> GHMG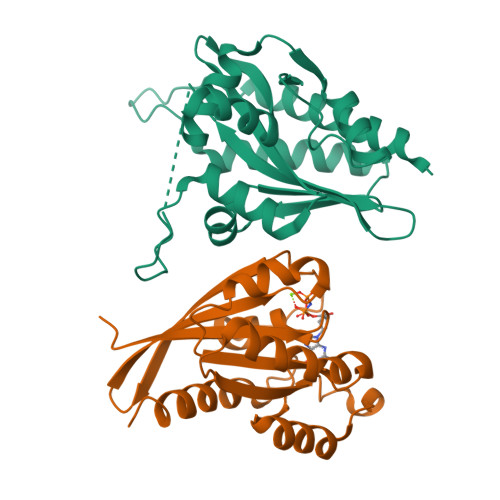QKASQQLALKDSKEVPVVCEVVSEAIVHAAQKLKEYLGFEYPPSKLCPAANTLNEIFLIHFITFCQEKGVDEWLTTTKMTKHQAFLFGADWIWTFWGSDKQIKLQLAVQTLQMSSPPPVESKPCDLSNPESRVEESSWKKSRFDKLEEFCNLIGEDCLGLFIIFGMPGKPKDIRGVVLDSVKSQMVRSHLPGGKAVAQFVLETEDCVFIKELLRNCLSKKDGLREVGKVYISIL;> MAHHHHHHSSGASAQDARYGQKDSSDQNFDYMFKLLIIGNSSVGKTSFLFRYADDSFTSAFVSTVGIDFKVKTVFKNEKRIKLQIWDTAGQERYRTITTAYYRGAMGFILMYDITNEESFNAVQDWSTQIKTYSWDNAQVILVGNKCDMEDERVISTERGQHLGEQLGFEFFETSAKDNINVKQTFERLVDIICDKMSESLETDPAITAAKQNTRLKETPPPPHPNCGC>[2x]MKKRIVLNAFDMTCVSHQSAGTWRHPSSQAARYNDLEYWTNMAMELERGCFDCLFIADVVGVYDVYRGSAEMALRDADQVPVNDPFGAISAMAAVTEHVGFGVTAAITFEQPYLLARRLSTLDHLTKGRVAWNVVSSYLNSAALNIGMDQQLA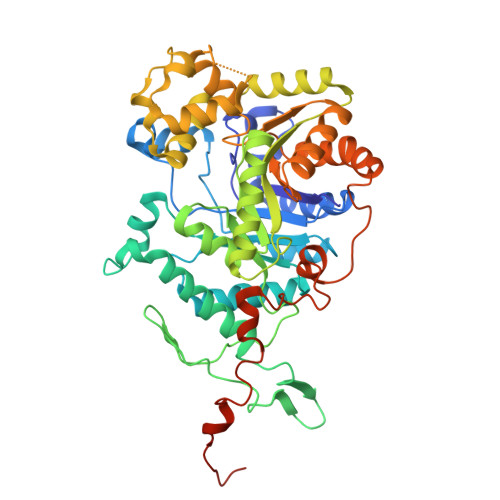HDERYEMADEYMEVMYKLWEGSWEDDAVKRDKKSGVFTDGSKVHPINHQGKYYKVPGFHICEPSPQRTPVIFQAGASGRGSKFAASNAEGMFILTTSVEQARQITTDIRNQAEAAGRSRDSIKIFMLLTVITGDSDEAAEAKYQEYLSYANPEGMLALYGGWTGIDFAKLDPDEPLQAMENDSLRTTLESLTHGENAKKWTVRDVIRERCIGGLGPVLVGGPQKVADELERWVDEGGVDGFNLAYAVTPGSVTDFIDYIVPELRKRGRAQDSYKPGSLRRKLIGTNDGRVESTHPAAQYRDAYVGKESVADRTQPSPFANAKAPVAELEHHHHHH>SLDKLHVTSTRPQYVRIKNWGSGEILHDTLHHKATSDFTCKSKSCLGSIMNPKSLTRGPRDKPTPLEELLPHAIEFINQYYGSFKEAKIEEHLARLEAVTKEIETTGTYQLTLDELIFATKMAWRNAPRCIGRIQWSNLQVFDARNCSTAQEMFQHICRHILYATNNGNIRSAITVFPQRSDGKHDFRLWNSQLIRYAGYQMPDGTIRGDAATLEFTQLCIDLGWKPRYGRFDVLPLVLQADGQDPEVFEIPPDLVLEVTMEHPKYEWFQELGLKWYALPAVANMLLEVGGLEFPACPFNGWYMGTEIGVRDFCDTQRYNILEEVGRRMGLETHTLASLWKDRAVTEINVAVLHSFQKQNVTIMDHHTASESFMKHMQNEYRARGGCPADWIWLVPPVSGSITPVFHQEMLNYVLSPFYYYQIEPW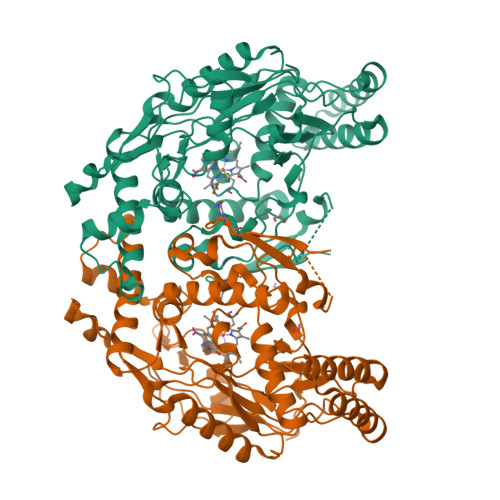KTHIWQNE[2x]> MAKDIEISASESKFILEALRQNYRLDGRSFDQFRDVEITFGKEFGDVSVKMGNTKVHCRISCQIAQPYEDRPFEGLFVISTEISPMAGSQFENGNITGEDEVLCSRIIEKSVRRSGALDVEGLCIVAGSKCWAVRADVHFLDCDGGFIDASCIAVMAGLMHFKKPDITVHGEQIIVHPVNEREPVPLGILHIPICVTFSFFNPQDTEENIKGETNSEISIIDATLKEELLRDGVLTVTLNKNREVVQVSKAGGLPMDALTLMKCCHEAYSIIEKITDQILQLLKEDSEKRNKYAAMLTSENAREI;> MSRLEIYSPEGLRLDGRRWNELRRFESSINTHPHAADGSSYMEQGNNKIITLVKGPKEPRLKSQMDTSKALLNVSVNITKFSKFERSKSSHKNERRVLEIQTSLVRMFEKNVMLNIYPRTVIDIEIHVLEQDGGIMGSLINGITLALIDAGISMFDYISGISVGLYDTTPLLDTNSLEENAMSTVTLGVVGKSEKLSLLLVEDKIPLDRLENVLAIGIAGAHRVRDLMDEELRKHAQKRVSNASAR;> MAESTTLETIEIHPITFPPEVLARISPELSLQRHLSLGIRPCLRKYEEFRDVAIENNTLSRYADAGNIDTKNNILGSNVLKSGKTIVITSITGGIIEETSAAIKDLDDFGEEELFEVTKEE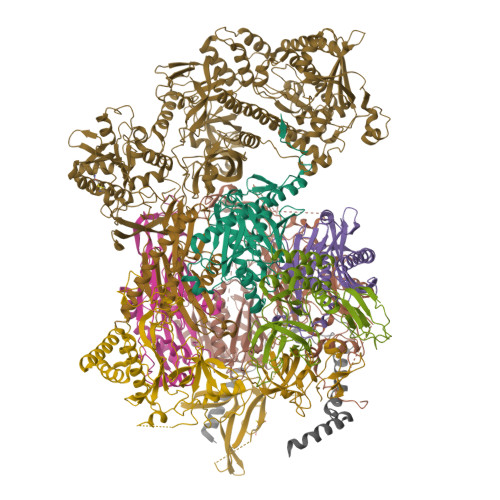DIIANYASVYPVVEVERGRVGACTDEEMTISQKLHDSILHSRILPKKALKVKAGVRSANEDGTFSVLYPDELEDDTLNETNLKMKRKWSYVLYAKIVVLSRTGPVFDLCWNSLMYALQSVKLPRAFIDERASDLRMTIRTRGRSATIRETYEIICDQTKSVPLMINAKNIAFASNYGIVELDPECQLQNSDNSEEEEVDIDMDKLNTVLIADLDTEAEETSIHSTISILAAPSGNYKQLTLMGGGAKITPEMIKRSLLLSRVRADDLSTRFNI;> MSVQAEIGILDHVDGSSEFVSQDTKVICSVTGPIEPKARQELPTQLALEIIVRPAKGVATTREKVLEDKLRAVLTPLITRHCYPRQLCQITCQILESGEDEAEFSLRELSCCINAAFLALVDAGIALNSMCASIPIAIIKDTSDIIVDPTAEQLKISLSVHTLALEFVNGGKVVKNVLLLDSNGDFNEDQLFSLLELGEQKCQELVTNIRRIIQDNISPRLVV;> MSLSVAEKSYLYDSLASTPSIRPDGRLPHQFRPIEIFTDFLPSSNGSSRIIASDGSECIVSIKSKVVDHHVENELLQVDVDIAGQRDDALVVETITSLLNKVLKSGSGVDSSKLQLTKKYSFKIFVDVLVISSHSHPISLISFAIYSALNSTYLPKLISAFDDLEVEELPTFHDYDMVKLDINPPLVFILAVVGNNMLLDPAANESEVANNGLIISWSNGKITSPIRSVALNDSNVKSFKPHLLKQGLAMVEKYAPDVVRSLENL;> MNVQDRRRLLGPAAAKPMAFSNTTTHVPEKKSTDLTPKGNESEQELSLHTGFIENCNGSALVEARSLGHQTSLISAVYGPRSIRGSFTSQGTISIQLKNGLLEKYNTNELKEVSSFLMGIFNSVVNLSRYPKSGIDIFVYLTYDKDLTNNPQDDDSQSKMMSSQISSLIPHCITSITLALADAGIELVDMAGAGEANGTVVSFIKNGEEIVGFWKDDGDDEDLLECLDRCKEQYNRYRDLMISCLMNQET;> MSTFIFPGDSFPVDPTTPVKLGPGIYCDPNTQEIRPVNTGVLHVSAKGKSGVQTAYIDYSSKRYIPSVNDFVIGVIIGTFSDSYKVSLQNFSSSVSLSYMAFPNASKKNRPTLQVGDLVYARVCTAEKELEAEIECFDSTTGRDAGFGILEDGMIIDVNLNFARQLLFNNDFPLLKVLAAHTKFEVAIGLNGKIWVKCEELSNTLACYRTIMECCQKNDTAAFKDIAKRQFKEILTVKEE;> MSEVITITKRNGAFQNSSNLSYNNTGISDDENDEEDIYMHDVNSASKSESDSQIVTPGELVTDDPIWMRGHGTYFLDNMTYSSVAGTVSRVNRLLSVIPLKGRYAPETGDHVVGRIAEVGNKRWKVDIGGKQHAVLMLGSVNLPGGILRRKSESDELQMRSFLKEGDLLNAEVQSLFQDGSASLHTRSLKYGKLRNGMFCQVPSSLIVRAKNHTHNLPGNITVVLGVNGYIWLRKTSQMDLARDTPSANNSSSIKSTGPTGAVSLNPSITRLEEESSWQIYSDENDPSISNNIRQAICRYANVIKALAFCEIGITQQRIVSAYEASMVYSNVGELIEKNVMESIGSDILTAEKMRGNGN;> MACNFQFPEIAYPGKLICPQYGTENKDGEDIIFNYVPGPGTKLIQYEHNGRTLEAITATLVGTVRCEEEKKTDQEEEREGTDQSTEEEKSVDASPNDVTRRTVKNILVSVLPGTEKGRKTNKYANNDFANNLPKEGDIVLTRVTRLSLQRANVEILAVEDKPSPIDSGIGSNGSGIVAAGGGSGAATFSVSQASSDLGETFRGIIRSQDVRSTDRDRVKVIECFKPGDIVRAQVLSLGDGTNYYLTTARNDLGVVFARAANGAGGLMYATDWQMMTSPVTGATEKRKCAKPF;> MSVPAIAPRRKRLADGLSVTQKVFVRSRNGGATKIVREHYLRSDIPCLSRSCTKCPQIVVPDAQNELPKFILSDSPLELSAPIGKHYVVLDTNVVLQAIDLLENPNCFFDVIVPQIVLDEVRNKSYPVYTRLRTLCRDSDDHKRFIVFHNEFSEHTFVERLPNETINDRNNRAIRKTCQWYSEHLKPYDINVVLVTNDRLNREAATKEVESNIITKSLVQYIELLPNADDIRDSIPQMDSFDKDLERDTFSDFTFPEYYSTARVMGGLKNGVLYQGNIQISEYNFLEGSVSLPRFSKPVLIVGQKNLNRAFNGDQVIVELLPQSEWKAPSSIVLDSEHFDVNDNPDIEAGDDDDNNESSSNTTVISDKQRRLLAKDAMIAQRSKKIQPTAKVVYIQRRSWRQYVGQLAPSSVDPQSSSTQNVFVILMDKCLPKVRIRTRRAAELLDKRIVISIDSWPTTHKYPLGHFVRDLGTIESAQAETEALLLEHDVEYRPFSKKVLECLPAEGHDWKAPTKLDDPEAVSKDPLLTKRKDLRDKLICSIDPPGCVDINDALHAKKLPNGNWEVGVHIADVTHFVKPGTALDAEGAARGTSVYLVDKRIDMLPMLLGTDLCSLKPYVDRFAFSVIWELDDSANIVNVNFMKSVIRSREAFSYEQAQLRIDDKTQNDELTMGMRALLKLSVKLKQKRLEAGALNLASPEVKVHMDSETSDPNEVEIKKLLATNSLVEEFMLLANISVARKIYDAFPQTAMLRRHAAPPSTNFEILNEMLNTRKNMSISLESSKALADSLDRCVDPEDPYFNTLVRIMSTRCMMAAQYFYSGAYSYPDFRHYGLAVDIYTHFTSPIRRYCDVVAHRQLAGAIGYEPLSLTHRDKNKMDMICRNINRKHRNAQFAGRASIEYYVGQVMRNNESTETGYVIKVFNNGIVVLVPKFGVEGLIRLDNLTEDPNSAAFDEVEYKLTFVPTNSDKPRDVYVFDKVEVQVRSVMDPITSKRKAELLLK;> MSLLEQLARKRIEKSKGLLSADQSHSTSKSASLLERLHKNRETKDNNAETKRKDLKTLLAKDKVKRSDFTPNQHSVSLSLKLSALKKSNSDLEKQGKSVTLDSKENELPTKRKSPDDKLNLEESWKAIKEMNHYCFLKNDPCINQTDDFAFTNFIIKDKKNSLSTSIPLSSQNSSFLSLKKHNNELLGIFVPCNLPKTTRKVAIENFNRPSPDDIIQSAQLNAFNEKLENLNIKSVPKAEKKEPINLQTPPTESIDIHSFIATHPLNLTCLFLGDTNAGKSTLLGHLLYDLNEISMSSMRELQKKSSNLDPSSSNSFKVILDNTKTERENGFSMFKKVIQVENDLLPPSSTLTLIDTPGSIKYFNKETLNSILTFDPEVYVLVIDCNYDSWEKSLDGPNNQIYEILKVISYLNKNSACKKHLIILLNKADLISWDKHRLEMIQSELNYVLKENFQWTDAEFQFIPCSGLLGSNLNKTENITKSKYKSEFDSINYVPEWYEGPTFFSQLYLLVEHNMNKIETTLEEPFVGTILQSSVLQPIAEINYVSLKVLINSGYIQSGQTIEIHTQYEDFHYYGIVSRMKNSKQILETNTKNNISVGLNPDILEVLVKIHNTEDFTKKQFHIRKGDIIIHSRKTNTLSPNLPNTLKLLALRLIKLSIQTHALSDPVDLGSELLLYHNLTHNAVKLVKILGTNDISINPNQSLIVEVEIIEPDFALNVIDSKYITNNIVLTSIDHKVIAVGRIACQ>MSKQELDAALKKAKELASSAPVVVFSKTYCGYCNRVKQLLTQVGASYKVVELDELSDGSQLQSALAHW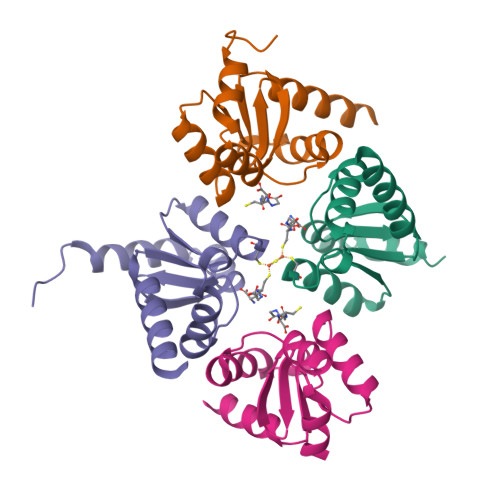TGRGTVPNVFIGGKQIGGCDTVVEKHQRNELLPLLQDAAATAKTSAQL[4x]> CSCSSLMDKECVYFCHLDIIW;> EERGFPPDRATPLLQTAEIMTPPTKTLWPKGDYKDDDDKLAPAEVPKGDRTAGSPPRTISPPPCQGPIEIKETFKYINTVVSCLVFVLGIIGNSTLLRIIYKNKCMRNGPNILIASLALGDLLHIVIDIPINVYKLLAEDWPFGAEMCKLVPFIQKASVGITVLSLCALSIDRYRAVASWSRIKGIGVPKWTAVEIVLIWVVSVVLAVPEAIGFDIITMDYKGSYLRICLLHPVQKTAFMQFYKTAKDWWLFSFYFCLPLAITAFFYTLMTCEMLRKKSGMQIALNDHLKQRREVAKTVFCLVLVFALCWLPLHLSRILKLTLYNQNDPNRCELLSFLLVLDYIGINMASLNSCINPIALYLVSKRFKNCFKSCLCCWCQSFEEKQSLEEKQSCLKFKANDHGYDNFRSSNKYSSSGSGGGGSGGSSSGGVFTLEDFVGDWEQTAAYNLDQVLEQGGVSSLLQNLAVSVTPIQRIVRSGENALKI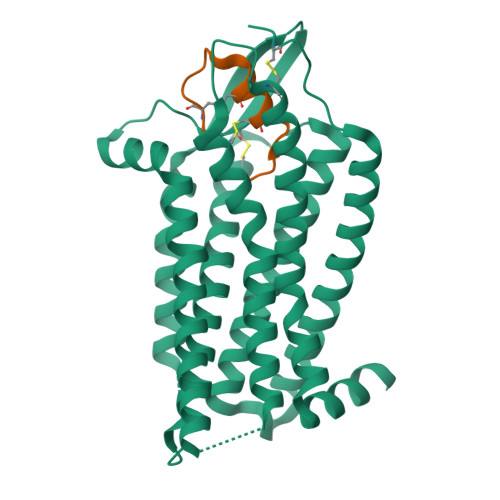DIHVIIPYEGLSADQMAQIEEVFKVVYPVDDHHFKVILPYGTLVIDGVTPNMLNYFGRPYEGIAVFDGKKITVTGTLWNGNKIIDERLITPDGSMLFRVTINSGGSGGGGSGGSSSGGLEVLFQ>[6x]DYYFDSYDHYGIHEEMLQDTVRTLSYRNAIIQNKDLFKDKIVLDVGCGTGILSMFAAKHGAKHVIGVDMSSIIEM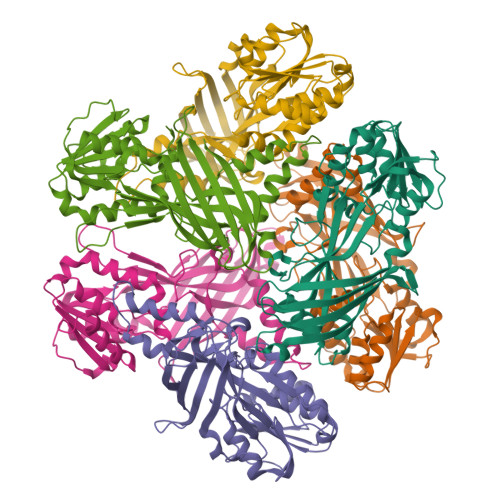AKELVELNGFSDKITLLRGKLEDVHLPFPKVDIIISEWMGYFLLYESMMDTVLYARDHYLVEGGLIFPDKCSIHLAGLEDSQYKDEKLNYWQDVYGFDYSPFVPLVLHEPIVDTVERNNVNTTSDKLIEFDLNTVKISDLAFKSNFKLTAKRQDMINGIVTWFDIVFPAPKGKRPVEFSTGPHAPYTHWKQTIFYFPDDLDAETGDTIEGELVCSPNEKNNRDLNIKISYKFESNGIDGNSRSRKNEGSYLMH>[6x]MGSSHHHHHHSQDPMLSKDIIKLLNEQVNKEMNSSNLYMSMSSWCYTHSLDGAGLFLFDHAAEEYEHA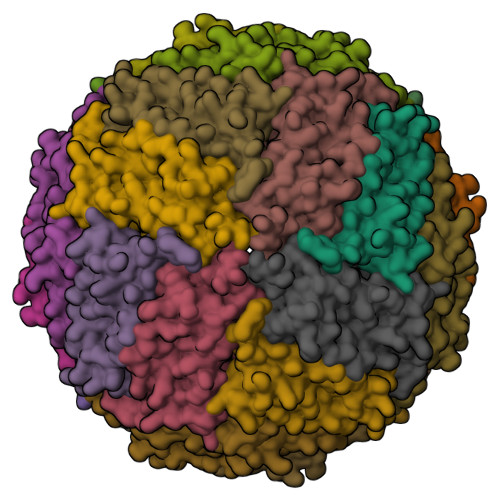KKLIIFLNENNVPVQLTSISAPEHKFEGLTQIFQKAYEHEQHISESINNIVDHAIKSKDHATFNFLQWYVAEQHEEEVLFKDILDKIELIGNENHGLYLADQYVKGIAKSRKS> SSLGSQKERLLDELTLEGVARYMQSERCRRVICLVGAGISTSAGIPDFRSPSTGLYDNLEKYHLPYPEAIFEISYFKKHPEPFFALAKELYPGQFKPTICHYFMRLLKDKGLLLRCYTQNIDTLERIAGLEQEDLVEAHGTFYTSHCVSASCRHEYPLSWMKEKIFSEVTPKCENCQSLVKPDIVFFGESLPARFFSCMQSDFLKVDLLLVMGTSLQVQPFASLISKAPLSTPRLLINKEKAGQSDPFLGMIMGLGGGMDFDS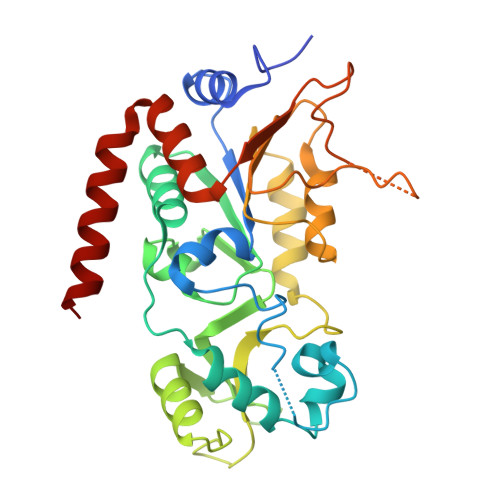KKAYRDVAWLGECDQGCLALAELLGWKKELEDLVRREHASIDAQ>[2x]MSALTSQGGRDMIPPEGKCNDHNSAFDFKLYMIRKAESVNAALDVSVPLREPLTVQEAVRYSLLAGGKRVRPLLCIA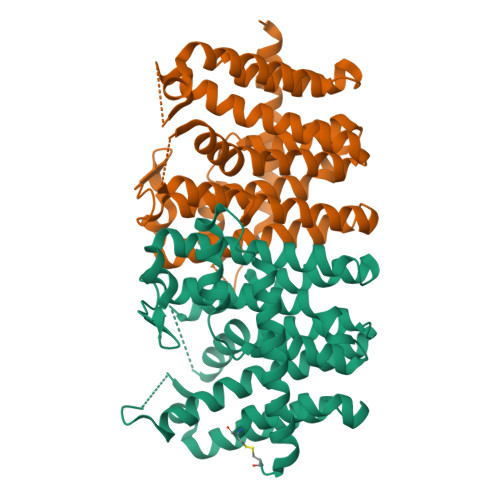VCELVGGDEATAMSAACAVEMIHTSSLIHDDLPCMDNADLRRGKPTNHKVYGEDMAVLAGDALLALAFEHMTVVSSGLVAPERMIRAVVELARAIGTTGLVAGQMIDLASERLNPDKVGLEHLEFIHLHKTAALLEAAAVLGVIMGGGTEEEIEKLRKYARCIGLLFQVVDDILDVTKSTEELGKTAGKDVMAGKLTYPRLIGLERSKEVAEKLRREAEEQLLGFDPSKAAPLVALASYIACRHNLEHHHHHH> MASVHGTTYELLRRQGIDTVFGNPGTNELPFLKDFPEDFRYILALQEACVVGIADGYAQASRKPAFINLHSAAGTGNAMGALSNAWNSHSPLIVTAGQQTRAMIGVEALLTNVDAANLPRPLVKWSYEPASAAEVPHAMSRAIHMASMAPQGPVYLSVPYDDWDKDADPQSHHLFDRHVSSSVRLNDQDLDILVKALNSASNPAIVLGPDVDAANANADCVMLAERLKAPVWVAPSAPRCPFPTRHPCFRGLMPAGIAAISQLLEGHDVVLVIGAPVFRYHQYDPGQYLKPGTRLISVTCDPLEAARAPMGDAIVADIGAMASALANLVEESSRQLPTAAPEPAKVDQDAGRLHPETVFDTLNDMAPENAIYLNESTSTTAQMWQRLNMRNPGSYYFCAAG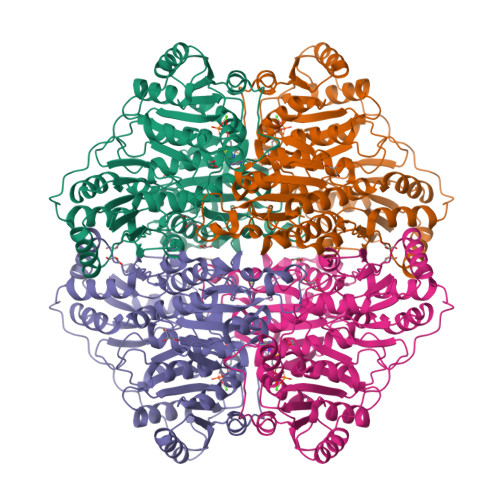GLGFALPAAIGVQLAEPERQVIAVIGDGSANYSISALWTAAQYNIPTIFVIMNNGTYGALRWFAGVLEAENVPGLDVPGIDFRALAKGYGVQALKADNLEQLKGSLQEALSAKGPVLIEVSTVSPVKHHHHHH> SMGVRKLATIRTAGEITPIAGAEAIECCHVDGWTCVIKKGEFKQGDRGVYFEIDSFIKEDNDRYPMLSKQVIDYEGQRGTRLRTARLRGQLSQGLFLPMDRFPELASNQVGDDVTEILGITKWEPPISTNLSGEILGEFPTFISKTDQERVQNLIPQIEENKGQKFEVTVKLDGSSMTVYRKDDHIGVCGRNWELRETATNAQWHAARRNKMIEGLQFLNRNLALQGEIIGESIQGNLEKLKGQDFYLFDIYDIDKAQYLTPIERQSLVKQLNDNGFTVKHVPILDDLELNHTAEQILAMADGPSLNKNVKREGLVFKRLDGKFSFA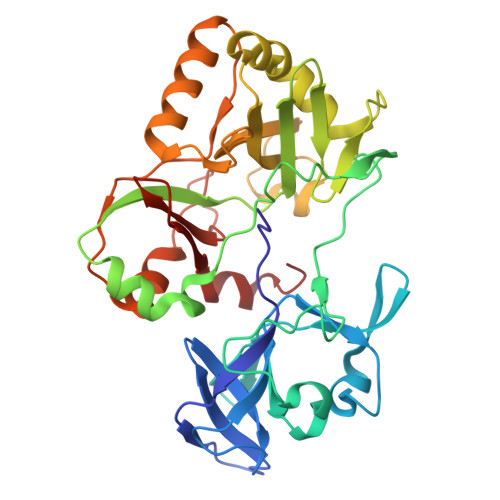AISNAYLEKHKDR>[2x]GPGSMTETTTTFMDNVLGWLH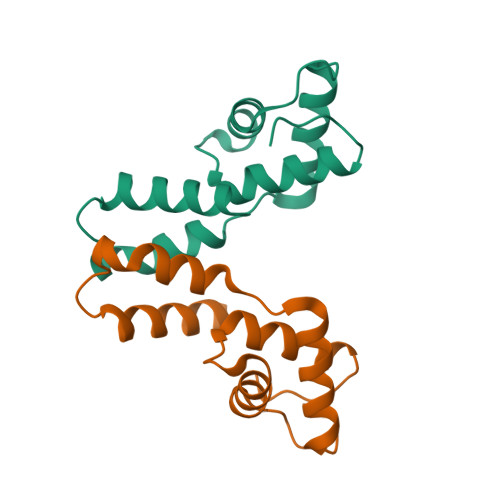KGYPEGVPPKDYFALLALLKRSLTEDEVVRAAQAILRSTDGQSPVTDDDIRNAVHQIIEKEPTAEEINQVAARLASVGWPLAVPVR The widespread and highly conserved ParDE TA systems, part of the RelE/ParE superfamily, target DNA gyrase. M. tuberculosis encodes two ParDE systems and several studies on the ParE1 and ParE2 toxins have shown their ability to inhibit gyrase enzymes from E. coli, M. smegmatis and M. tuberculosis. Toxin-antitoxin (TA) systems are found in most bacterial genomes and generally comprise small bicistronic loci encoding a protein toxin and a protein or RNA antitoxin. Here, we present microbiological, biochemical, structural and biophysical characterisation of the ParDE1 and ParDE2 TA systems from M. tuberculosis.

Single datasets were collected from 3 crystals and subsequently merged to a final resolution of 2.10 Å. The ParDE1 complex revealed in the crystal structure is of a ParD14ParE12 heterohexamer, with two full-length (‘primary’) ParD1 antitoxins resolved alongside two shorter, partially resolved (‘auxiliary’), ParD1 antitoxins. The ParE1 toxin is comprised of α1 (P9–W26), α2 (V28–A47), α3 (P49–I51), β1 (R61–A67), β2 (H70–T77), β3 (G80–H89) and α4 (Q90–M92), with 3 C-terminal residues unresolved. α1 and α2 form a hairpin-like structure as a base. The primary ParD1 protomers are comprised of β1 (T5–V8), α1 (E13–A23), α2 (A29–S60), α3 (F68–S80). The auxiliary ParD1 protomer secondary structures are the same as the primary ParD1 protomers from residues G2–E55, with the C-terminal A56–R83 unresolved. The heterohexameric structure somewhat resembles the search model, with the ParD1 antitoxins interacting via an anti-parallel N-terminal β sheet (though noting only one pair of the antiparallel β sheets was resolved), and a pair of ParE1 toxins positioned inside a cage-like structure. A coiled-coil interaction is present, however, between helix α2 of the primary ParD1 chains and helix α2 of the auxiliary ParD1 chains, forming alongside the anti-parallel β sheet that is itself part of a ribbon-helix-helix (RHH) DNA binding motif. Mapping these to the surface of the ParE1 toxin shows two highly conserved hydrophobic patches used as binding sites for a single ParD1 primary chain; one site along the groove created by the antiparallel β strands (1–3), and the other site on the underside of the toxin structure between the hairpin of α helices 1 and 2, as also picked out by PISA. ParD1 antitoxin binds to these patches similarly to how ParD2 was observed binding ParE2, though it is notable that ParE1 does not encode the proposed C-terminal helix in ParE2 that is displaced by ParD2. Remodelling allows conversion of two ParDE1 heterotetramer complexes into a single heterohexameric complex, and for every heterohexamer produced two ParE1 toxin molecules are liberated.

>[2x]MSSRYLLSPAAQAHLEEIWDCTYDRWGVDQAEQYLRELQHAIDRAAANPRIGRACDEIRPGYRKLSAGSHTLFYRVTGEGTIDVVRVLHQRMDVDRNL;>MGKNTSFVLDEHYSAFIDGEIAAGRYRSASEVIRSALRLLEDRETQLRALREALEAGERSGSSTPFDFDGFLGRKRADASRGR[4x]(2~{E},5~{R},10~{E},12~{E},15~{S},19~{R})-20-[[(2~{R},3~{R})-3-aminocarbonyloxy-2-methyl-butanoyl]amino]-3,5,15-trimethyl-7-methylidene-19-oxidanyl-17-oxidanylidene-icosa-2,10,12-trienoic acid 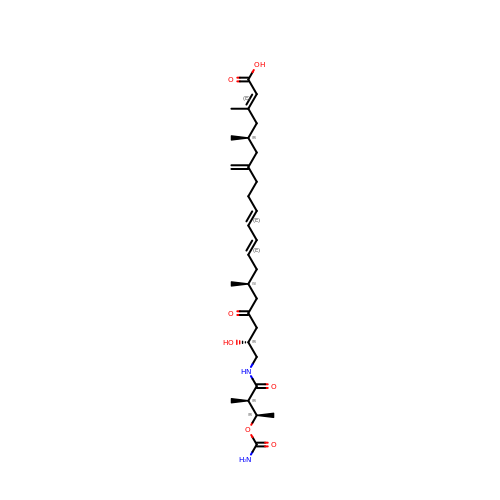| C30 H48 N2 O7 | GENAAYFYLGYPIQ-YPMJEBJESA-N> ISGGDAIYSSTGRCSLGFNVRSGSTYYFLTAGHCTDGATTWWANSARTTVLGTTSGSSFPNNDYGIVRYTNTTIPKDGTVGGQDITSAANATVGMAVTRRGSTTGTHSGSVTALNATVNYGGGDVVYGMIRTNVCAEPGDSG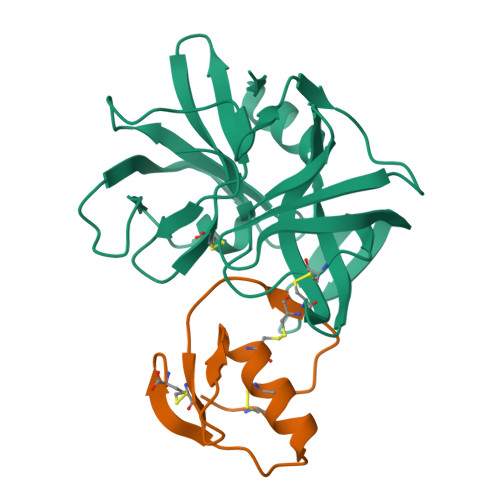GPLYSGTRAIGLTSGGSGNCSSGGTTFFQPVTEALVAYGVSVY;> VDCSEYPKPACTTEYRPLCGSDNKTYGNKCNFCNAVVESNGTLTLSHFGKC>[3x]MKIHPTAIIDPKAELHESVEVGPYSIIEGNVSIQEGTIIEGHVKICAGSEIGKFNRFHQGAVIGVMPQDLGFNQQLLTKTVIGDHNIFREYSNIHKGTKEDSPTVIGNKNYFMGNSHVGHDCILGNNNILTHGAVLAGHVTLGNFAFISGLVAVHQFCFVGDYSMVAGLAKVVQDVPPYSTVDGNPSTVVGLNSVGMKRAGFSPEVRNAIKH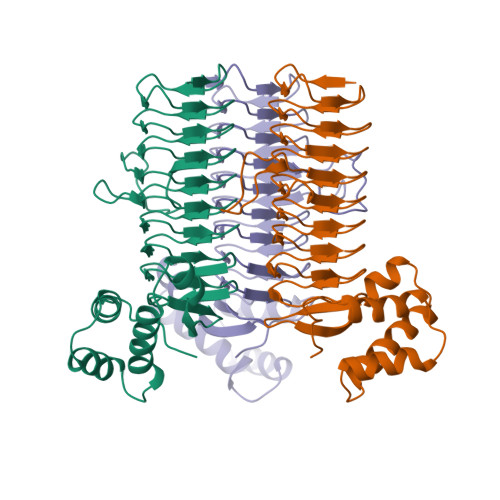AYKVIYHSGISTRKALDELEASGNLIEQVKYIIKFFRDSDRGVTNHR> MQSMILFAAALMGAAVNGFVLPRTDDPDCETKATDCGSTSNIKYTVVKGDTLTSIAKKFKSGICNIVSVNKLANPNLIELGATLIIPENCSNPDNKSCVSTPAEPTETCVPGLPGSYTIVSGDTLTNISQDFNITLDSLIAANTQIENPDAIDVGQIITVPVCPSSQCEAVGTYNIVAGDLFVDLAATYHTTIGQIKALNNNVNPSKLKVGQQIIL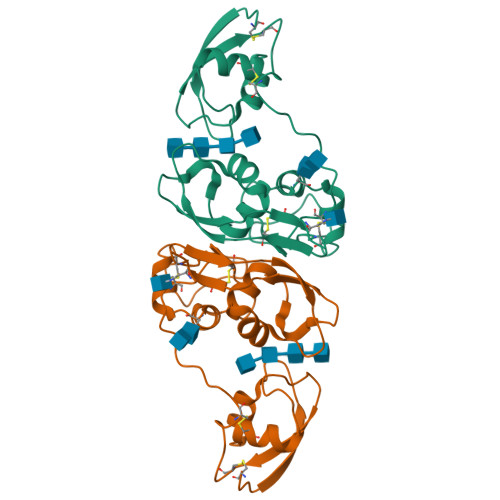PQDCKNVTTAVA>[4x]MSLADDLKIALIYGKTGPLEAYAKQTETGLMMGLEYATKGTMTLDGRKIVVITKDDQSKPDLSKAALAEAYQDDGADIAIGTSSSAAALADLPVAEENKKILIVEPAVADQITGEKWNRYIFRTGRNSSQDAISNAVAIGKQGVTIATLAQDYAFGRDGVAAFKEALAKTGATLA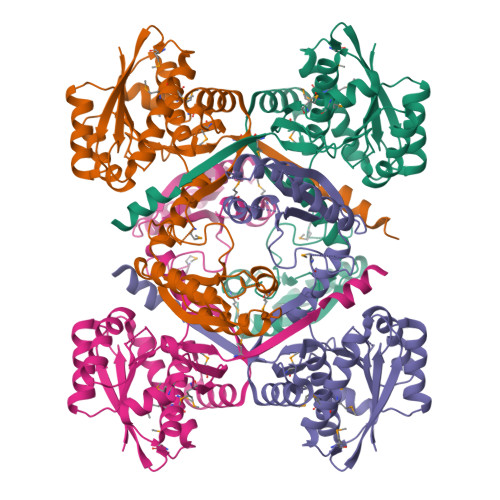TEEYVPTTTTDFTAVGQRLFDALKDKPGKKIIWVIWAGGGDPLTKLQDMDPKRYGIELSTGGNILPALAAYKRLPGMEGATYYYYDIPKNPINEWLVTEHQKRFNAPPDFFTAGGFSAAMAVVTAVQKAKSTDTEKLIAAMEGMEFDTPKGKMVFRKEDHQALQSMYHFKVKVDPAVAWAVLEEGHHHHHH>QLTTESMPFNVAEGKEVLLLVHNLPQQLFGYSWYKGERVDGNRQIVGYAIGTQQATPGPANSGRETIYPNASLLIQNVTQNDTGFYTLQVIKSDLVNEE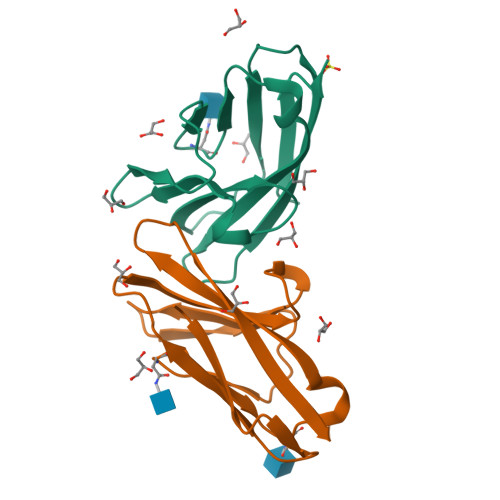ATGQFHVY[2x]> MNDIAHNLAQVRDKISAAATRCGRSP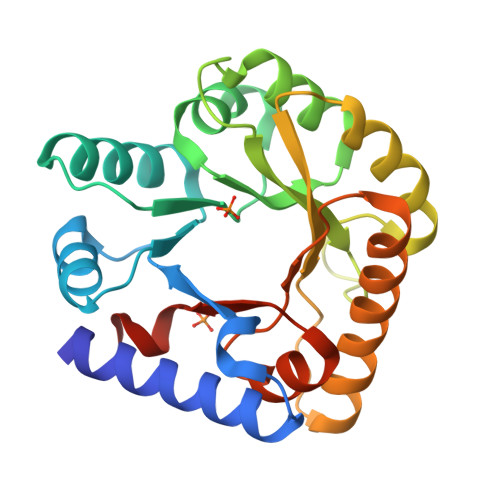EEITLLAVSATAPASAIAEAIDAGQRQFGENYVQEGVDKIRHFQELGVTGLEWHFIGPLQSNKSRLVAEHFDWCHTIDRLRIATRLNDQRPAELPPLNVLIQINISDENSKSGIQLAELDELAAAVAELPRLRLRGLMAIPAPESEYVRQFEVARQMAVAFAGLKTRYPHIDTLSLGMSDDMEAAIAAGSTMVRIGTAIFGARDYSKK>MMANRMILNETAWFGRGAVGALTDEVKRRGYQKALIVTDKTLVQCGVVAKVTDKMDAAGLAWAIYDGVVPNPT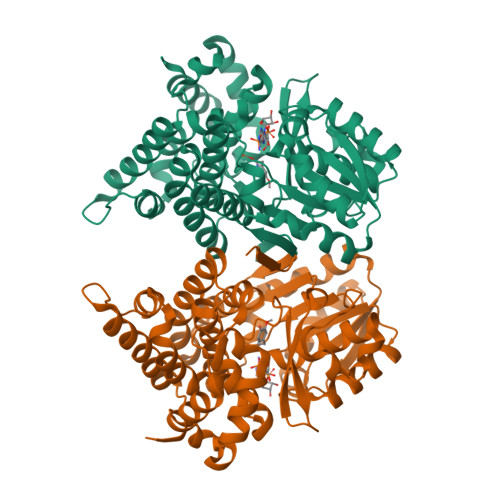ITVVKEGLGVFQNSGADYLIAIGGGSPQDTCKAIGIISNNPEFADVRSLEGLSPTNKPSVPILAIPTTAGTAAEVTIGYVITDEEKRRKFVCVDPHDIPQVAFIDADMMDGMPPALKAATGVDALTHAIEGYITRGAWALTDALHIKAIEIIAGALRGSVAGDKDAGEEMALGQYVAGMGFSNVGVGLVHGMAHPLGAFYNTPHGVANAILLPHVMRYNADFTGEKYRDIARVMGVKVEGMGLEEARNAAVEAVFALNRDVGIPPHLRDVGVRKEDIPALAQAALDDVCTGGNPREATLEDIVELYHTAWTSHHHHH[2x]>[2x]GHMRELQADFVKPARIDILLDMPPASRDLQLKHSWNSEDRSLNIFVKEDDKLTFHRHPVAQSTDCI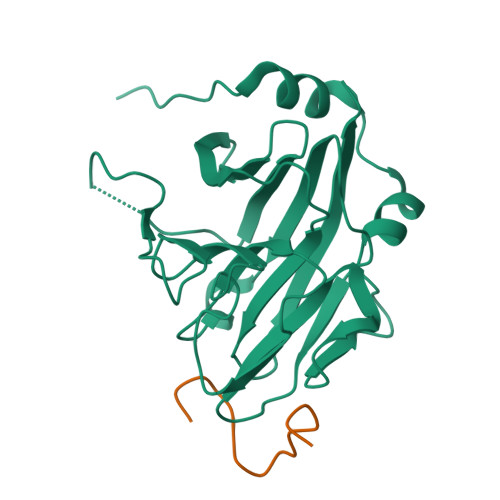RGKVGLTKGLHIWEIYWPTRQRGTHAVVGVCTADAPLHSVGYQSLVGSTEQSWGWDLGRNKLYHDSKNCAGVTYPAILKNDEAFLVPDKFLVALDMDEGTLSFIVDQQYLGIAFRGLRGKKLYPIVSAVWGHCEITMRYIGGLVDELN;>[2x]DINNNNNIVEDVERKREFYI> SIDDIDELIQDMEIKE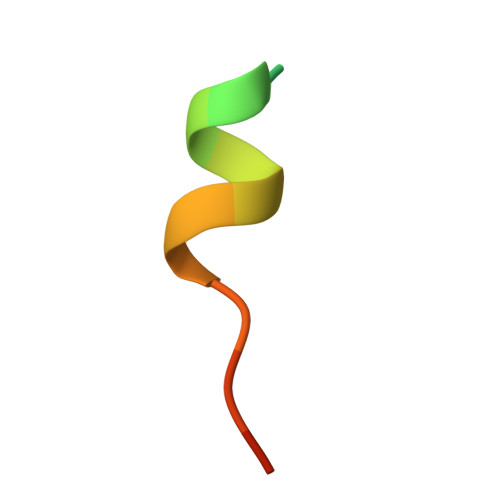E>GPLGNPPAEVSTSLKVYQGHTLEKTYMGEDFFWAITPTAGDYILFKFDKPVNVESYLFH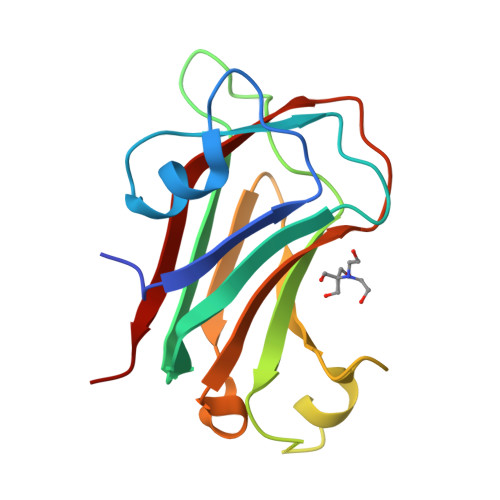SGNQEHPGAILLNTTVDVLPLKSDSLEISKETKDKRLEDGYFRIGKFEYGVAEGIVDPGLNPISAFRLSVIQNSAVWAILNEIHIKKVTS[6x]> HHHHHHTDPQGDAAQKTDTSHHDQDHPTFNKITPNLAEFAFSLYRQLAHQSNSTNIFFSPVSIATAFAMLSLGTKADTHDEILEGLNFNLTEIPEAQIHEGFQELLRTLNQPDSQLQLTTGNGLFLSEGLKLVDKFLEDVKKLYHSEAFTVNFGDTEEAKKQINDYVEK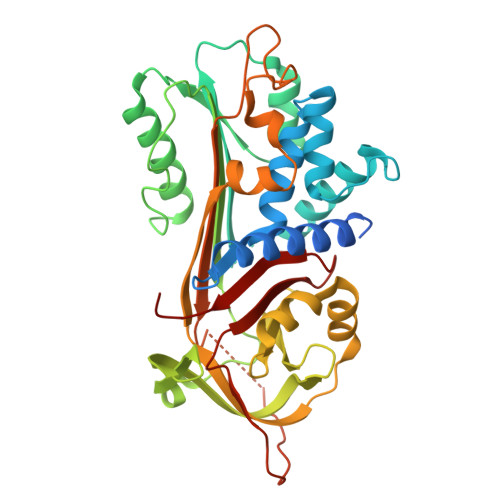GTQGKIVDLVKELDRDTVFALVNYIFFKCKWERPFEVKDTEEEDFHVDQVTTVKVPMMKRLGMFNIQHCKKLSSWVLLMKYLGNATAIFFLPDEGKLQHLENELTHDIITKFLENEDRRSASLHLPKLSITGTYDLKSVLGQLGITKVFSNGADLSGVTEEAPLKLSKAVHKAVLTIDEKGTEAAGAMFLEAIPMSIPPEVKFNKPFVFLMIEQNTKSPLFMGKVVNPTQK>[3x]PLYECQTVKGTLSERQRQSLAESITSIHTRETGAPASYVHVLFKEL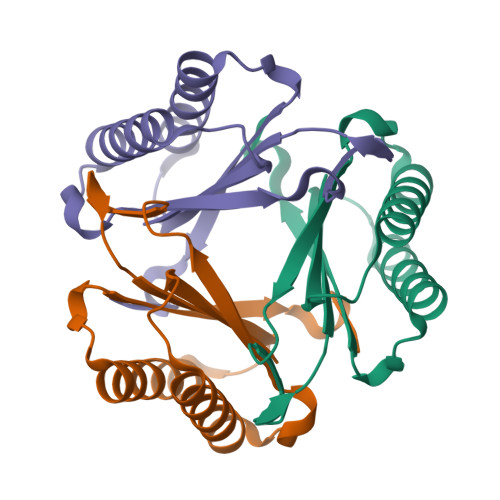EPGSAFTAGQVATPAIIRGQIRAGRPQATRHAILRAITDVYMAVTGADANAVVVAVVDIPASWAMEGGQIFPEPEQPPEVA> QGAMEVLDINDNEPVFTQDVFVG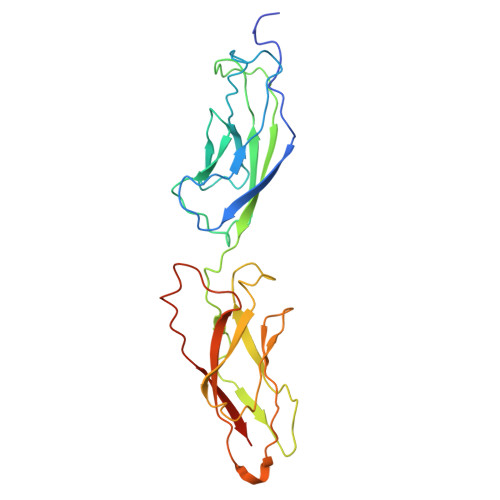SVEELSAAHTLVMKINATDADEPNTLNSKISYRIVSLEPAYPPVFYLNKDTGEIYTTSVTLDREEHSSYTLTVEARDGNGEVTDKPVKQAQVQIRILDVNDNIPVVENKVLEGMVEENQVNVEVTRIKVFDADEIGSDNWLANFTFASGNEGGYFHIETDAQTNEGIVTLIKEVDYEEMKNLDFSVIVANKAAFHKSIRSKYKPTPIPIKVKVKNVKEGI>[180x]MEIYEGKLTAEGLRFGIVASRFNHALVDRLVEGAIDCIVRHGGREEDITLVRVPGSWEIPVAAGELARKEDIDAVIAIGVLIEGAEPHFDYIA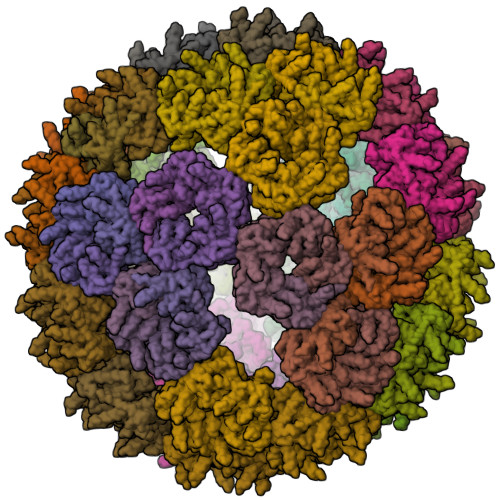SEVSKGLANLSLELRKPITFGVITADELEEAIERAGTKHGNKGWEAALSAIEMANLFKSLRLEHHHHH> HGSPVDICTAKPRDIPMNPMCIYRSPEKKATEDEGSEQKIPEATNRRVWELSKANSRFATTFYQHLADSKNDNDNIFLSPLSISTAFAMTKLGACNDTLQQLME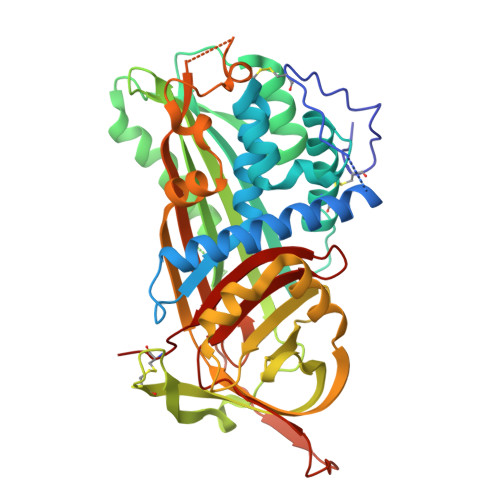VFKFDTISEKTSDQIHFFFAKLNCRLYRKANKASKLVSANRLFGDKSLTFNETYQDISELVYGAKLQPLDFKENAEQSRAAINKWVSNKTEGRITDVIPSEAINVLVLVNTRTSTVLVLVNTIYFKGLWKSKFSPENTRKELFYKADGESCSASMMYQEGKFRYRRVAEGTQVLELPFKGDDITMVLILPKPEKSLAKVEKELTPEVLQEWLDELEEMMLVVHMPRFRIEDGFSLKEQLQDMGLVDLFSPEKSKLPGIVAEGRDDLYVSDAFHKAFLEVNEEGSEAAASTAVVIAGRSLNPNRVTFKANRPFLVFIREVPLNTIIFMGRVANPCVK> XCVIFPVEIDVSQTIIRDCQVDKQTRELVYINKIMNTQLTKPVLMMFNISGPIRSVTRKNNNLRDRIKSKVDEQFDQLERDYSDQMDGFHDSIK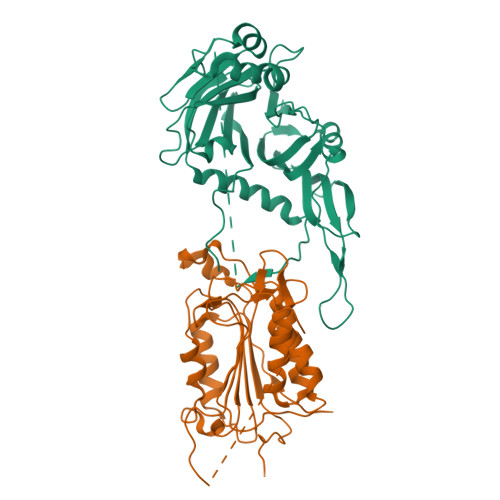YFKDEHYSVSCQNGSVLKSKFAKILKSHDYTDKKSIEAYEKYCLPKLVDERNDYYVAVCVLKPGFENGSNQVLSFEYNPIGNKVIVPFAHEINDTGLYEYDVVAYVDSVQFDGEQFEEFVQSLILPSSFKNSEKVLYYNEASKNKSMIYKALEFTTESSWGKSEKYNWKIFCNGFIYDKKSKVLYVKLHNVTSALNKNVILNTIK;> LDKVYQMKSKPRGYCLIINNHNFAKAREKVPKLHSIRDRNGTHLDAGALTTTFEELHFEIKPHHDCTVEQIYEILKIYQLMDHSNMDCFICCILSHGDKGIIYGTDGQEAPIYELTSQFTGLKCPSLAGKPKVFFIQACQGDNYQKGIPVETDSEEQPYLEMDLSSPQTRYIPDEADFLLGMATVNNCVSYRNPAEGTWYIQSLCQSLRERCPRGDDILTILTEVNYEVSNKDDKKNMGKQMPQPTFTLRKKLVFPSD>[2x]GPMELAHREYQAGDFEAAERHCMQLWRQEPDNTGVLLLLSSIHFQCRRLDRSAHFSTLAIKQNPLLAEAYSNLGNVYKERGQLQEAIEHYR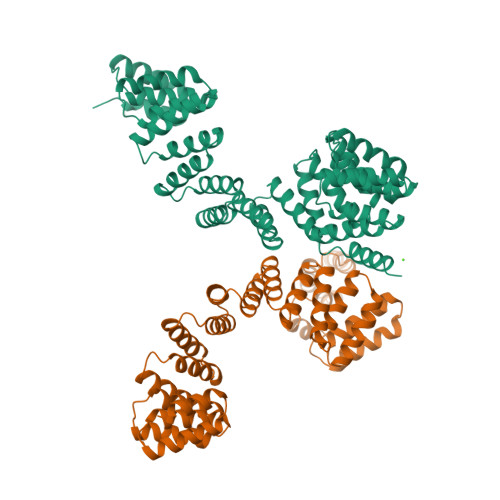HALRLKPDFIDGYINLAAALVAAGDMEGAVQAYVSALQYNPDLYCVRSDLGNLLKALGRLEEAKACYLKAIETQPNFAVAWSNLGCVFNAQGEIWLAIHHFEKAVTLDPNFLDAYINLGNVLKEARIFDRAVAAYLRALSLSPNHAVVHGNLACVYYEQGLIDLAIDTYRRAIELQPHFPDAYCNLANALKEKGSVAEAEDCYNTALRLCPTHADSLNNLANIKREQGNIEEAVRLYRKALEVFPEFAAAHSNLASVLQQQGKLQEALMHYKEAIRISPTFADAYSNMGNTLKEMQD> SNAKNVELTEKPESPVSINKTIKKSDIEDKGNKEEKNTVNYETVNKKAPIINVYNHITGKTEKMDMENYLCGVLAGEMSSEFDIEALKAQSVAARTYVVYKQEHGKSSKHKNAVVCTDYKHCQEYKSYDTLKKLN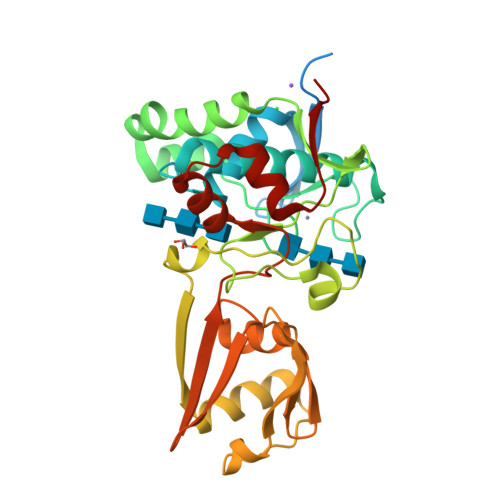GEEWIKNKYSKIQEAVRGTKGQIITYNDKAILPLYFSTSSGKTENSEEVFSAKYPYLKSVESPYDKYSPKFASTLKISNTDFVKSLRRAYSTIVIDVNNLSKQVSITKRSDAGTVEKIKLGNKELTGKDIRTVFKLNSANFDIKFGEGYIDFVVKGYGHGVGMSQWGAEGMAEEGYKYYDILSHYYTDTKIKDIY1-{[(3S,4S)-3-(3-fluorophenyl)-4-{[4-(1,3,4-triethyl-1H-pyrazol-5-yl)piperidin-1-yl]methyl}pyrrolidin-1-yl]methyl}cyclopentane-1-carboxylic 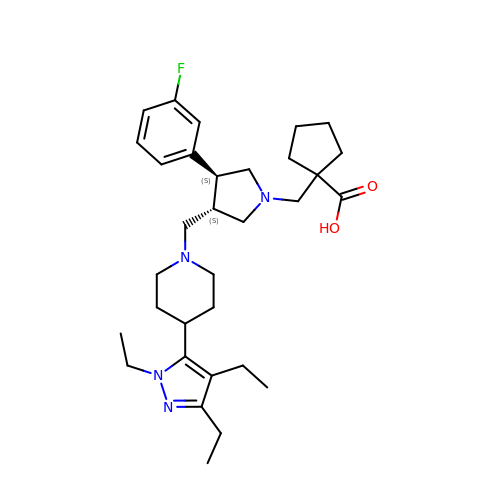acid | C32 H47 F N4 O2 | PCCHYTAFAXFIAW-LBNVMWSVSA-N> SMAMKATRLAIPDVILFEPRVFGDDRGFFFESYNQRAFEEACGHPVSFVQD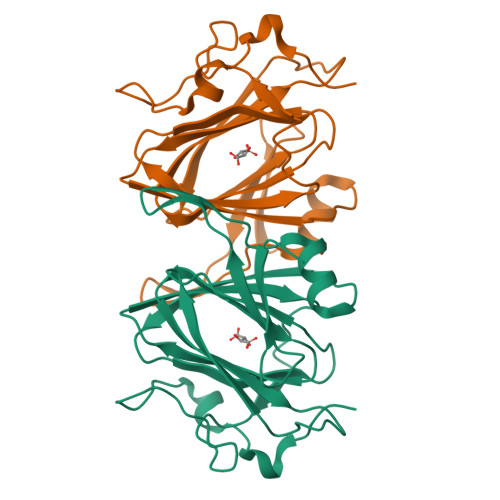NHSRSARGVLRGLHYQIRQAQGKLVRATLGEVFDVAVDLRRGSPTFGQWVGERLSAENKRQMWIPAGFAHGFVVLSEYAEFLYKTTDFWAPEHERCIVWNDPELKIDWPLQDAPLLSEKDRQGKAFADADCFP> GLTEEQKQEIREAFDLFDTDGSGTIDAKELKVAMRALGFEPKKEEIKKMIADIDKDGSGTIDFEEFLQMMTAKMGERDS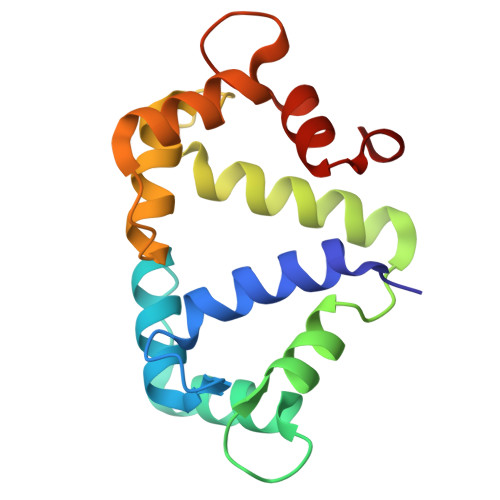REEIMKAFRLFDDDETGKISFKNLKRVAKELGENMTDEELQEMIDEADRDGDGEVNEEEFFRIMKKTSLF>[2x]MRGSHSGAQGLLAAQKARGLFKDFFPETGTKIELPELFDRGTASFPQTIYCGFDPTADSLHVGHLLALLGLFHLQRAGHNVIALVGGATARLGDPSGRTKEREALETERVRANARALRLGLEALAANHQQLFTDGRSWGSFTVLDNSAWYQKQHLVDFLAAVGGHFRMGTLLSRQSVQLRLKSPEGMSLAEFFYQVLQAYDFYYLFQRYGCRVQLGGS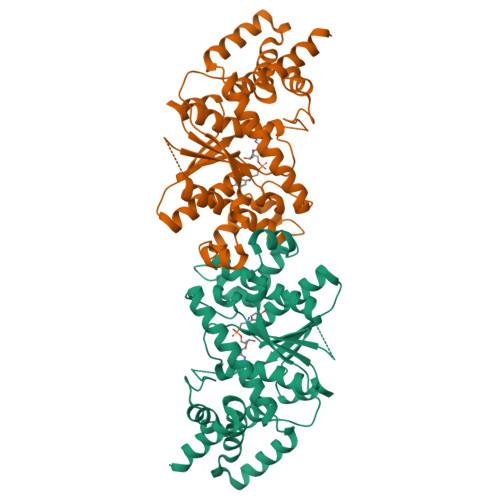DQLGNIMSGYEFINKLTGEDVFGITVPLITSTTGAKLGKSAGNAVWLNRDKTSPFELYQFFVRQPDDSVERYLKLFTFLPLPEIDHIMQLHVKEPERRGPQKRLAAEVTKLVHGREGLDSAKRCTQALYHRSHHHHHH>MGSSHHHHHHSSGLVPRGSHMASNSTYAPNVDSTVSLKGTDVFKADSASIAQNYTIPEWFKDAKFGIFIHWGVYSVPAYGSEWYSRWMYKEGHPINKYHVQTYGPLTKFGYKDFIPMFKAENFNADEWLAVVKSSGAQYIVPVAEHHDGFAMYSSTFNKWNAVDMGPKRDIIGELKEATKKAGLRFGLSSHRCENAWFYEYGMETPSDVQDTTITLYGERLHEPEGQGMTPYCGKYEGSNERSRRQFLMHTYELIDKYQPELIWFNWTVGKYPFQPTFYKFMAYYYNSALDWNKEVVVNTKFGYGDNIQVFDIERGKSDRIREYPWQTDTSVGKKSWSYCVGEENKSPDHIIDDFVDIVSKNGNLLLNIGPKADGTITDEQKNVLAEIGKWLKTNGEAIYGSRPWVIASEGHNAGTAGYMTDNTKTEYTADDIRFTTCDNNLYAVSLAWTDGSVTIKSLATKYCRNVEIESVEMLGSSEKIDYKMTDEGLVVNFPKNKPTEYAHVFKIKLKGVVVSKPLYDKVDNGCLITVRVANHNAEDANVTLKSVVDGNEVSTQVAVKAKSEQWVKMQNKDVKSFDDMSCKFYF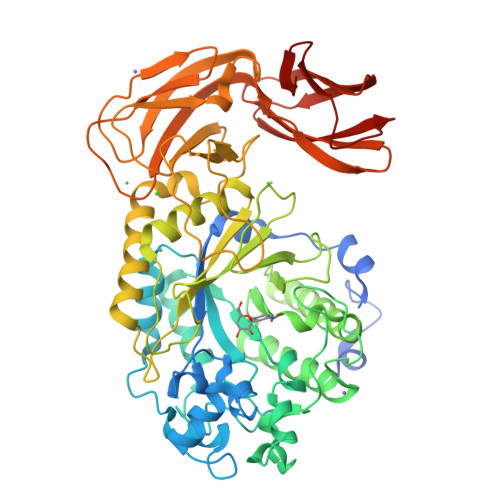NDNLTYENEFKK[4x]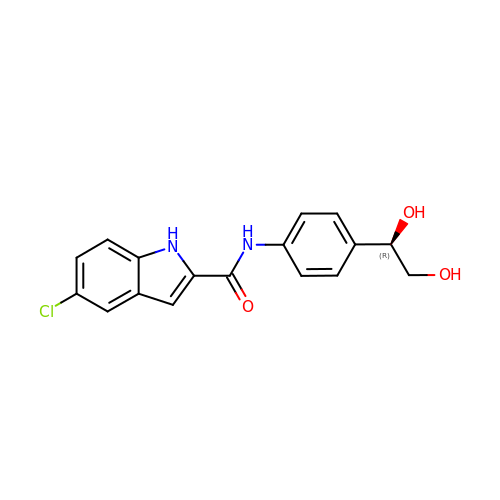5-chloro-N-{4-[(1R)-1,2-dihydroxyethyl]phenyl}-1H-indole-2-carboxamide | C17 H15 Cl N2 O3 | SHCHFGSUYJUEBR-INIZCTEOSA-N> KS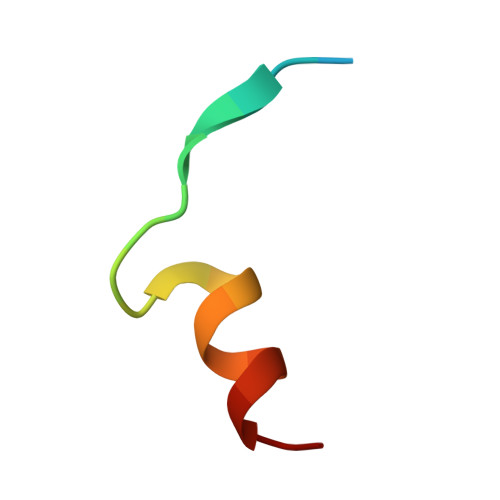LYKIKPRHDSGIKAKISMKT>MASSLAPRQVIRDGQFITSPNGKYKLVMQADGNLVLYEDGTKPIWNTTPVGPGAKAVMEFNLNLYNKAGQVAWSSNVYTAYLFEEFKDEAYLNLQDDGDFGIFSDEAKWGSIVLSRPEVGVKNKIIPTGTVMVPGTEYINGNYRLAFQGDGNLVIYQINPQVVIWATYTMGADRAVVQEDGNFVIYKGTTALWHTHTATGMPAYLKFTNTGKLFLSQPTLLWTLKRGSLSKPPKVIPGQHGPLDTTPIWSWPHDYPRRRAVVHHHHHH[2x]

Here we report on the discovery of a novel member of this family, pyocin L1 from P. aeruginosa, and show that it utilises lipopolysaccharide (LPS) as a surface receptor, specifically targeting the common polysaccharide antigen (CPA) that is a conserved homopolymer of d-rhamnose. Alignment of the pyocin L1 protein sequence with other lectin-like bacteriocins, LlpA1Pf-5, LlpAPss642, putidacin L1 (LlpABW), LlpAAu1504 from Burkholderia cenocepacia and LlpAXcm761 from Xanthomonas citri pv. malvacearum shows that pyocin L1 contains tandem MMBL domains with three conserved QxDxNxVxY MMBL sugar-binding motifs. Pyocin L1, as predicted by sequence homology to MMBL proteins, consists of two tandem β-prism domains characteristic of MMBLs, connected by antiparallel strands propagating from the end of each MMBL domain and lending a strand to the reciprocal β-prism. In this work we have shown that pyocin L1 targets susceptible cells through binding to the CPA component of LPS and that primary recognition of CPA occurs through binding of d-rhamnose at the conserved QxDxNxVxY sugar binding motifs of the C-terminal lectin domain.

In an attempt to determine the location of the pyocin L1 d-rhamnose binding site(s) and the structural basis of the d-rhamnose specificity of pyocin L1 we determined the X-ray structures of pyocin L1 with bound d-mannose, d-rhamnose and in the unbound form. The strands contain a tryptophan residue which forms π-stacking interactions with two other tryptophans in the β-prism to stabilise the structure. This interaction is conserved throughout MMBLs, with most members of the class utilising it to form either homo- or hetero-dimers of single MMBL subunits. However, in pyocin L1, as with the recently described structure of putidacin L1, both domains are from a single polypeptide chain. Other structural elements are also common between the two bacteriocins, namely a C-terminal extension of 30 amino acids and a two-turn α-helix insertion into loop 6 of the N-terminal MMBL domain. The overall root mean square deviation (rmsd) of backbone atoms for pyocin L1 and putidacin L1 is 7.5 Å, which is relatively high due to a difference in the relative orientation of the two MMBL domains. Comparison of the respective N- and C- terminal domains from pyocin L1 and putidacin L1 shows they possess very similar folds with rmsds of 2.77 Å and 2.02 Å, respectively. The higher value for comparison of the N-terminal domains is due to the presence of a 2-strand extension to β-sheet two of the putidacin L1 N-terminal MMBL domain, which is absent from pyocin L1 and other MMBLs. MMBL dimers of plant origin often form higher order structures, however small angle X-ray scattering of pyocin L1 showed it to be monomeric in solution.> VTSYTLSDVVSLKDVVPEWVRIGFSATTGAEYAAHEVLSWS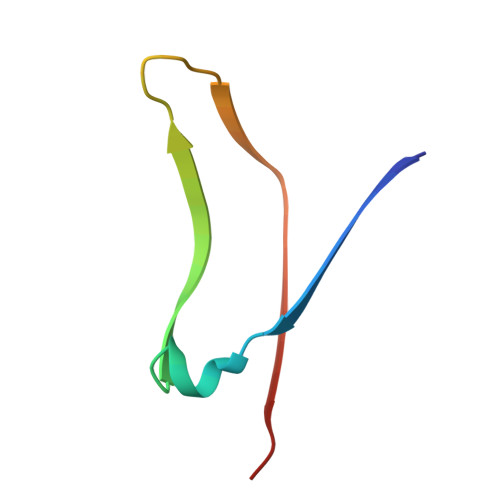FHSELSG>PKKIVKDAKEKLEKLLEDAKDGGEELALDIAEELAREAEKALKELLREGASPELIVDLAETALRALLEIAKDGGEELALDIARILAKLAEVALEVLLKDGASPKLIVDLAKTALRALLEIAEDGGEELALDIAEILAELAEVALRVLLKDGASPKLIEDLAKTALDALEEIARDGGEE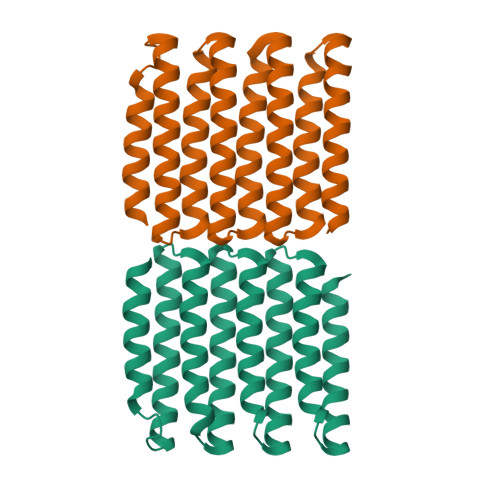LAEDIDRILRKLEKVARDVLRKDGAS[2x]> MGATKILMDSTHFNEIRSIIRSRSVAWDALARSEELSEIDASTAKALESILVKKNIGDGLSSSNNAHSGFKVNGKTLIPLIHLLSTSDNEDCKKSVQNLIAELLSSDKYGDDTVKFFQEDPKQLEQLFDVSLKGDFQTVLISGFNVVSLLVQNGLHNVKLVEKLLKNNNLINILQNIEQMDTCYVCIRLLQELAVIPEYRDVIWLHEKKFMPTLFKILQRATDSQLATRIVATNSNHLGIQLQYHSLLLIWLLTFNPVFANELVQKYLSDFLDLLKLVKITIKEKVSRLCISIILQCCSTRVKQHKKVIKQLLLLGNALPTVQSLSERKYSDEE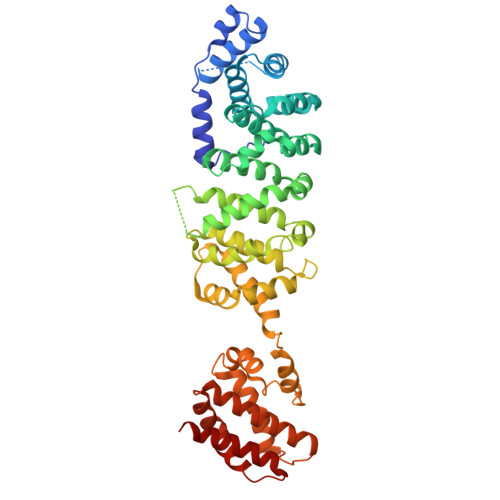LRQDISNLKEILENEYQELTSFDEYVAELDSKLLCWSPPHVDNGFWSDNIDEFKKDNYKIFRQLIELLQAKVRNGDVNAKQEKIIIQVALNDITHVVELLPESIDVLDKTGGKADIMELLNHSDSRVKYEALKATQAIIGYTFK>SMLKLSAENESTPIQQLLEHFLRQLQRKDPHGFFAFPVTDAIAPGYSMIIKH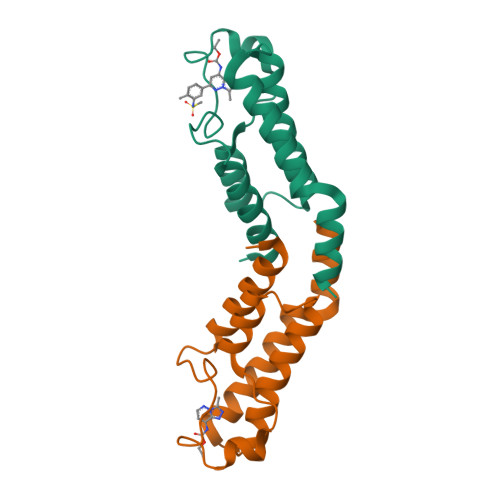PMDFGTMKDKIVANEYKSVTEFKADFKLMCDNAMTYNRPDTVYYKLAKKILHAGFKMMSKERLLALKRSMS[2x]> VLGGDECDINEHPFLAFLYSHGYFCGLTLINQEWVVTAAHCDSTNFQMQLGVHSKKVLNEDEQTRNPKEKFICPNKNMSEVLDKDIMLIKLDKPISNSKHIAPLSLPSNPPSVGSVCRIMGWGSITI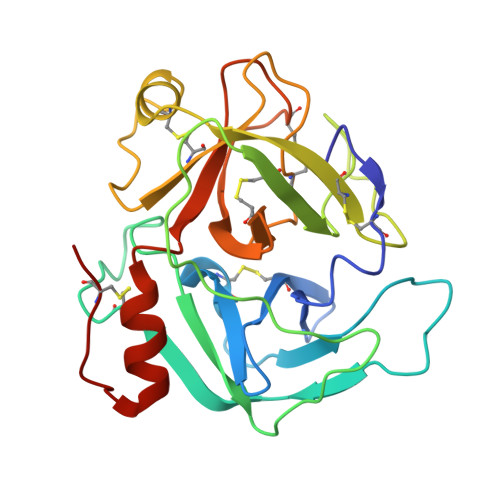PNETYPDVPYCANINLVDYEVCQGAYNGLPAKTTLCAGVLEGGKDTCVGDSGGPLICNGQFQGIVSYGAHSCGQGPKPGIYTNVFDYTDWIQRNIAGNTDATCPP> HHHHHHSEMTPREIVSELDKHIIGQDNAKRSVAIALRNRWRRMQLNEELRHEVTPKNILMIGPTGVGKTEIARRLAKLANAPFIKVEATKFTEVGYVGKEVDSIIRDLTDAAVKMVRVQAIEKNRYRAEELAEERILDVLIPPAKNNWGQTEQQQEPSAARQAFRKKLREGQLDDKEIEIDLAAAPMGVEIMAPPGMEEMTSQLQSMFQNL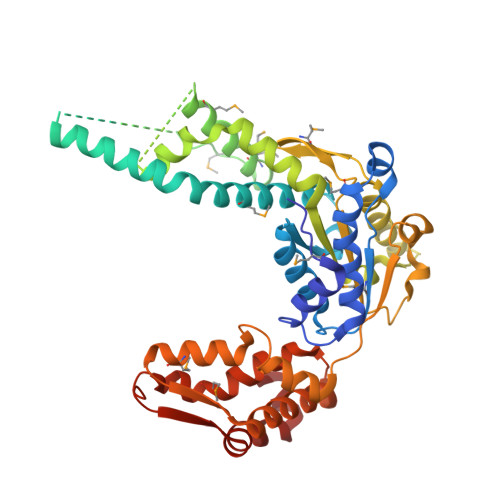GGQKQKARKLKIKDAMKLLIEEEAAKLVNPEELKQDAIDAVEQHGIVFIDEIDKICKRGESSGPDVSREGVQRDLLPLVEGCTVSTKHGMVKTDHILFIASGAFQIAKPSDLIPELQGRLPIRVELQALTTSDFERILTEPNASITVQYKALMATEGVNIEFTDSGIKRIAEAAWQVNESTENIGARRLHTVLERLMEEISYDASDLSGQNITIDADYVSKHLDALVADEDLSRFIL>[2x]GSAMGSSD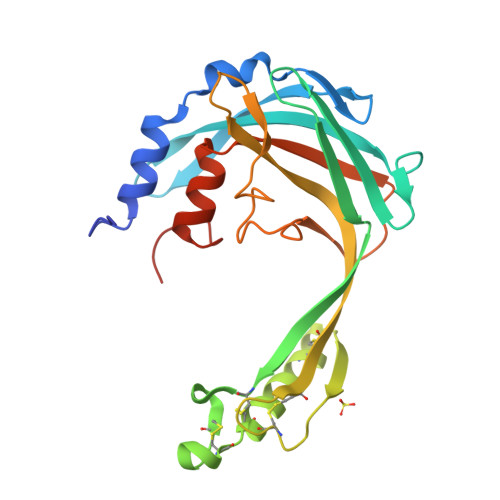DPRDNFKKAVSAFDPKPLESWTGTFSDVKATVRRQSLSVAGLGSIPSVYTEATVPVSGNTDGSQLVVKVNINTVAPFTRRSPLHATRERWFSCSSSQCSGYSRKCDCQEKHEQFRNKCYSQGGQYSTQSSKCRLGEKCGYCKQEVYLSKLYLVAASDGKGEYRESTQYQSALYSFGHLSQGYEAVPQDKVQVQLYSEGDPFIALERETMGEGEFGVPNRTAAA>GPLGSMFDIKRKTIEWGGKTLVLETGRIARQADGAVLATMGETVVLATAVFAKSQKPGQDFFPLTVNYQEKTFAAGKIPGGFFKREGRPSEKETLVSRLIDRPIRPLFVKGFKNEVQVVVTVLQHDLENDPDILGMVAASAALCLSGAPFMGPIGAARVGWVDGAYVLNPTLDEMKESKMDLVVAGTADAVMMVESEIQELSEEIVLGGVNFAHQQMQAVIDAIIDLAEHAAKEPFAFEPEDTDAIKAKMKDLVGADIAAAYKIQKKQDRYEAVGAAKKKAIAALGLSDENPTGYDPLKLGAIFKELEADVVRRGILDTGLRIDGRDVKTVRPILGEVGILPRTHGSALFTRGETQAIVVATLGTGDDEQFIDALEGTYKESFLLHYNFPPYSVGETGRMGSPGRREIGHGKLAWRALRPMLPTKEDFPYTIRLVSEITESNGSSSMATVCGS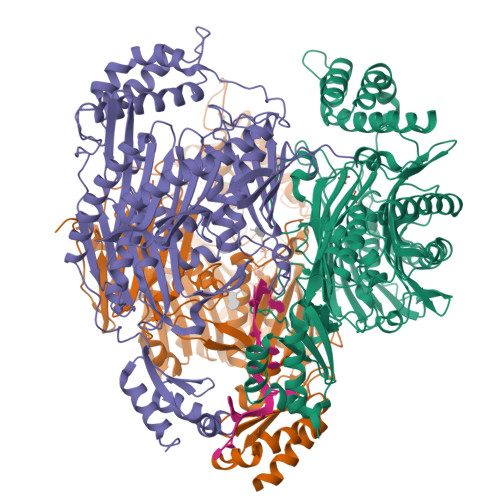SLAMMDAGVPLVRPVSGIAMGLILEQDGFAVLSDILGDEDHLGDMDFKVAGTSEGLTSLQMDIKIAGITPAIMEQALAQAKEGRAHILGEMNKAMDAPRADVGDFAPKIETINIPTDKIREVIGSGGKVIREIVATTGAKVDINDDGVVKVSASDGAKIKAAIDWIKSITDEAEVGKIYDGKVVKVVDFGAFVNFFGAKDGLVHVSQISNERVAKPSDVLKEGQMVKVKLLGFDDRGKTKLSMKVVDQETGEDLSKKEAAAEEA[3x]> PPYLKWA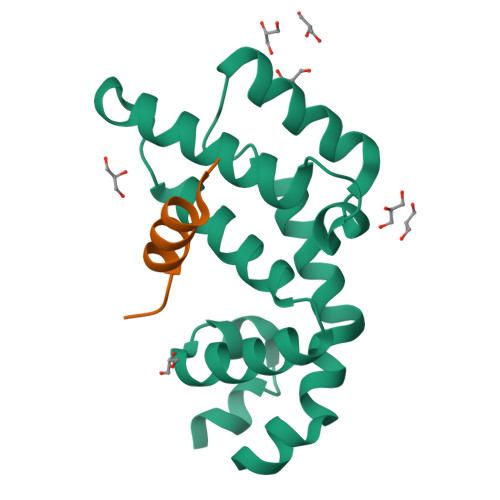ESLHSLLDDQDGISLFRTFLKQEGCADLLDFWFACTGFRKLEPCDSNEEKRLKLARAIYRKYILDNNGIVSRQTKPATKSFIKGCIMKQLIDPAMFDQAQTEIQATMEENTYPSFLKSDIYLEYT;> SEDDLLQECISSAMPK> GSMSGIALSRLAQERKAWRKDHPFGFVAVPTKNPDGTMNLMNWECAIPGKKG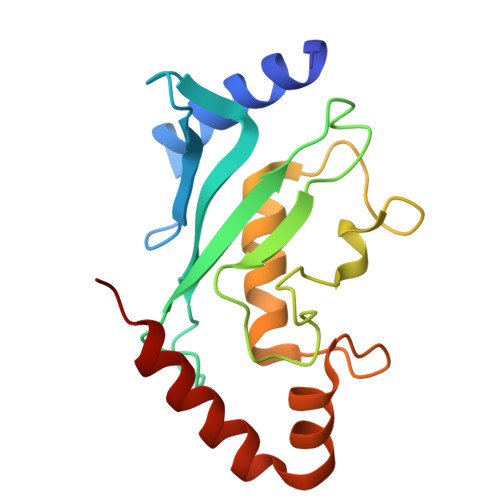TPWEGGLFKLRMLFKDDYPSSPPKCKFEPPLFHPNVYPSGTVCLSILEEDKDWRPAITIKQILLGIQELLNEPNIQDPAQAEAYTIYCQNRVEYEKRVRAQAKKFAPS>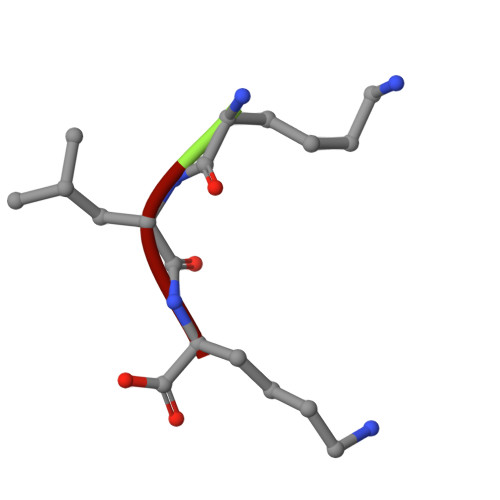 KLK>[8x]MMVISEKVRKALNDQLNREIYSSYLYLSMATYFDAEGFKGF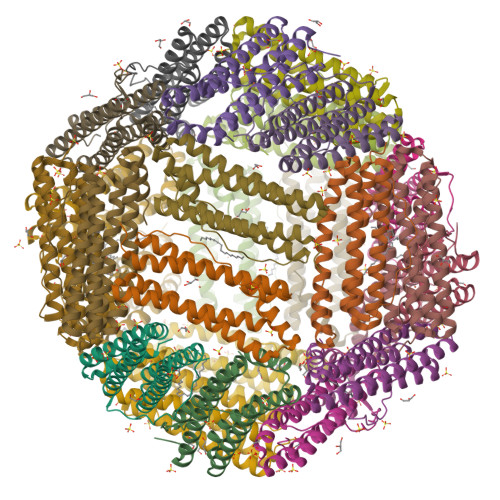AHWMKKQAQEELTHAMKFYEYIYQRGGRVELEAIEKPPSNWNGIKDAFEAALKHEEFVTQSIYNILELASEEKDHATVSFLKWFVDEQVEEEDQVREILDLLEKANGQMSVIFQLDRYLGQRE> MKEVARVRNLNRIIMGKYEIEPWYFSPYPIELTDEDF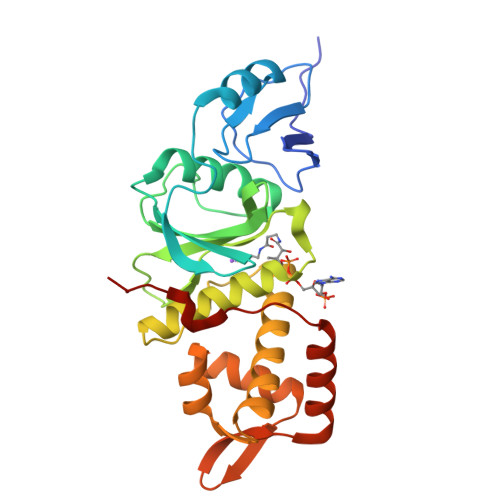IYIDDFTLQYFGSKKQYERYRKKCTLRHPPGNEIYRDDYVSFFEIDGRKQRTWCRNLCLLSKLFLDHKTLYYDVDPFLFYCMTRRDELGHHLVGYFSKEKESADGYNVASILTLPQYQRMGYGKLLIEFSYELSKKENKVGSPEKPLSDLGLLSYRAYWSDTLITLLVEHQKEITIDEISSMTSMTTTDILHTAKTLNILRYYKGQHIIFLNEDILDRYNRLKAKKRRTIDPNRLIWKPPV> ARKHVQELLKTFRRIDFDETRKSVYLQSAKFGVQSQLREPLTKKVLNYWDDVKLSKTCLDRMVTKVNDVKETFYAGFSYACESHNQYSVDCLEAAKPSYL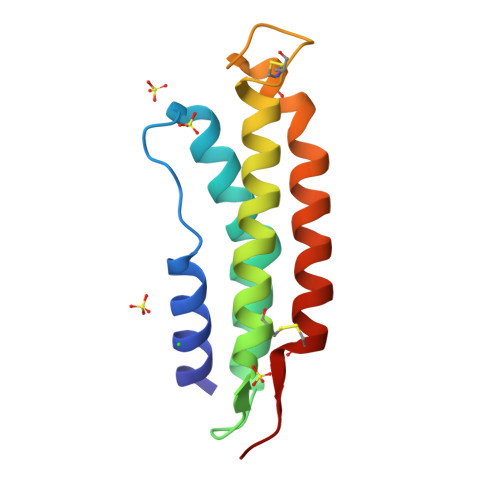TALGEIRGETEKCLTTRLK>[4x]ASMRPVRLMKVFVTRR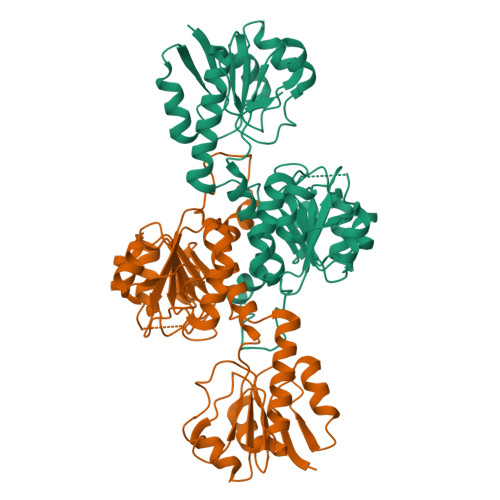IPAEGRVALARAADCEVEQWDSDEPIPAKELERGVAGAHGLLCLLSDHVDKRILDAAGANLKVISTMSVGIDHLALDEIKKRGIRVGYTPDVLTDTTAELAVSLLLTTCRRLPEAIEEVKNGGWTSWKPLWLCGYGLTQSTVGIIGLGRIGQAIARRLKPFGVQRFLYTGRQPRPEEAAEFQAEFVSTPELAAQSDFIVVACSLTPATEGLCNKDFFQKMKETAVFINISRGDVVNQDDLYQALASGKIAAAGLDVTSPEPLPTNHPLLTLKNCVILPHIGSATHRTRNTMSLLAANNLLAGLRGEPMPSELKL> GSHMLRLSAPGQLDDDLCLLGDVQVPVFLLRLGEASWALVEGGISRDAELVWADLCRWVADPSQVHYWLITHKHYDHCGLLPYLCPRLPNVQVLASERTCQAWKSESAVRVVERLNRQLLRAEQRLPEACAWDALPVRAVADGEWLELGPRHRLQVIEAHGHSDDHVVFYDVRRRRLFCG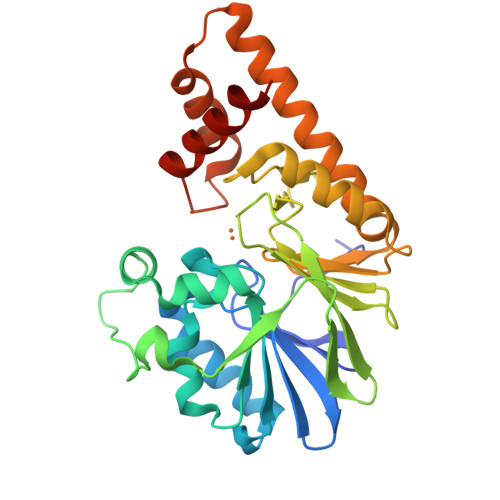DALGWFDEAEGVWRPLVFDDMEAYLESLERLQRLPTLLQLIPGHGGLLRGRLAADGAESAYTECLRLCRRLLWRQSMGESLDELSEELHRAWGGQSVDFLPGALHLGSMRRMLEILSRQALPLD>[2x]DIKVTPGTSELVEQILALLSRYLSSYIHVLNKFISHLRRVATLRFERTTL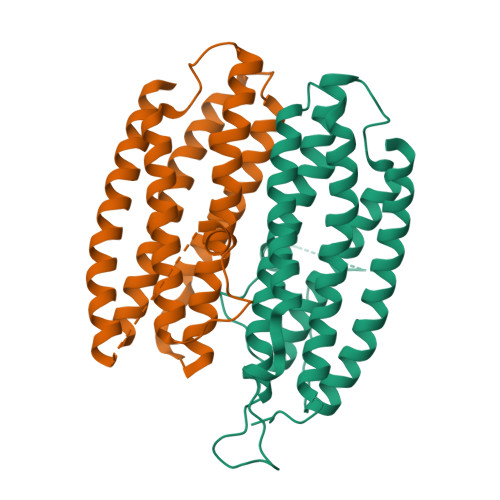IKFVKKLRFYNDSVLSYNASEFINEGKNELDPEADSFDKVILPIASMFVKSVETFDLLNYYLTQSLQKEILSKTLNEDLTLTAESILAIDDTYNHFVKFSQWMIESLRIGSNLLDLEVVQFAIKSADEDGTNIGETDNIFLQEILPVNSEEEFQTLSAAWHSILDGKLSALDEEFDVVATKWHD>[2x]SMAMQKIFAREILDSRGNPTVEVDLHTAKGRFRAAVPSGASTGIYEALELRDGDKGRYLGKGVLKAVENINSTLGPALLQKKLSVADQEKVDKFMIELDGTENKSKFGA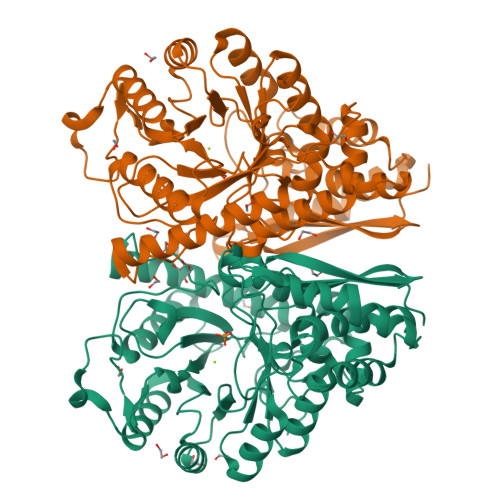NAILGVSLAVCKAGAAEKGVPLYRHIADLAGNPDLILPVPAFNVINGGSHAGNKLAMQEFMILPVGASSFKEAMRIGAEVYHHLKGVIKAKYGKDATNVGDEGGFAPNILENNEALELLKTAIQAAGYPDKVVIGMDVAASEFYRNGKYDLDFKSPDDPARHITGEKLGELYKSFIKNYPVVSIEDPFDQDDWATWTSFLSGVNIQIVGDDLTVTNPKRIAQAVEKKACNCLLLKVNQIGSVTESIQACKLAQSNGWGVMVSHRSGETEDTFIADLVVGLCTGQIKTGAPCRSERLAKYNQLMRIEEALGDKAIFAGRKFRNPKAK>ISEFGSSRMLTTLIYRSQVHPDRPPVDLDALVHRASSKNLPLGITGILLFNGLQFFQVLEGTEEALESLFSEIQSDPRHRDVVELMRDYSAYRRFHGTGMRILDLRLFETDGALEEILRFSTFGVTEPVNDRMFRLLSAFIADGGRYCLPEPLQPSRWMMMPASGTAAPQHLPGQPCQFALQAIVEPAKKRVSSFEALIRSPTGGSPVEMFAAIAAEDRYRFDLESKAYAFALAGQLPLGKHQLAINLLPGSLYHHPDAVGWLMDSLLAAGLRPDQVLIEVTETEVITCFDQFRKVLKALRVA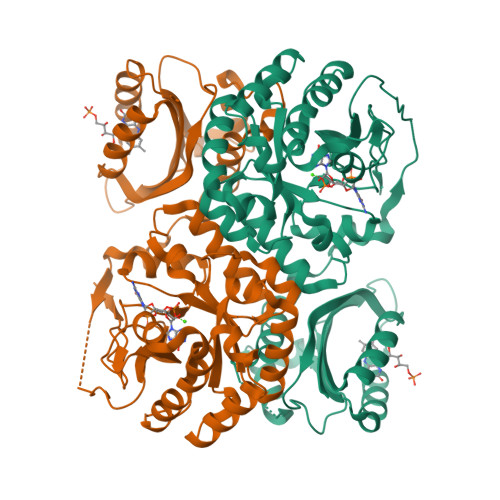GMKLAIDDFGAGYSGLSLLTRFQPDKIKVDAELVRDIHISGTKQAIVASVVRCCEDLGITVVAEGVETLEEWCWLQSVGIRLFQGFLFSRPCLNGIGEICWPVARQAMDL[2x]> MVALSLKISIGNVVKTMQFEPSTMVYDACRIIRERIPEAPAGPPSDFGLFLSDDDPKKGIWLEAG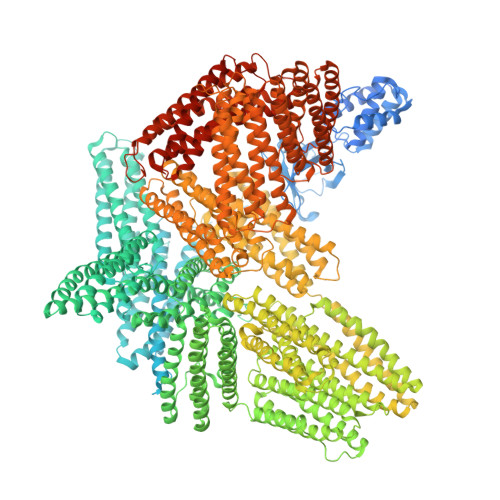KALDYYMLRNGDTMEYRKKQRPLKIRMLDGTVKTIMVDDSKTVTDMLMTICARIGITNHDEYSLVRELMEEKKEEITGTLRKDKTLLRDEKKMEKLKQKLHTDDELNWLDHGRTLREQGVEEHETLLLRRKFFYSDQNVDSRDPVQLNLLYVQARDDILNGSHPVSFDKACEFAGFQCQIQFGPHNEQKHKAGFLDLKDFLPKEYVKQKGERKIFQAHKNCGQMSEIEAKVRYVKLARSLKTYGVSFFLVKEKMKGKNKLVPRLLGITKECVMRVDEKTKEVIQEWNLTNIKRWAASPKSFTLDFGDYQDGYYSVQTTEGEQIAQLIAGYIDIILKKKKSKDHFGLEGDEESTMLEDSVSPKKSTVLQQQYNRVGKVEHGSVALPAIMRSGASGPENFQVGSMPPAQQQITSGQMHRGHMPPLTSAQQALTGTINSSMQAVQAAQATLDDFDTLPPLGQDAASKAWRKNKMDESKHEIHSQVDAITAGTASVVNLTAGDPAETDYTAVGCAVTTISSNLTEMSRGVKLLAALLEDEGGSGRPLLQAAKGLAGAVSELLRSAQPASAEPRQNLLQAAGNVGQASGELLQQIGESDTDPHFQDALMQLAKAVASAAAALVLKAKSVAQRTEDSGLQTQVIAAATQCALSTSQLVACTKVVAPTISSPVCQEQLVEAGRLVAKAVEGCVSASQAATEDGQLLRGVGAAATAVTQALNELLQHVKAHATGAGPAGRYDQATDTILTVTENIFSSMGDAGEMVRQARILAQATSDLVNAIKADAEGESDLENSRKLLSAAKILADATAKMVEAAKGAAAHPDSEEQQQRLREAAEGLRMATNAAAQNAIKKKLVQRLEHAAKQAAASATQTIAAAQHAASTPKASAGPQPLLVQSCKAVAEQIPLLVQGVRGSQAQPDSPSAQLALIAASQSFLQPGGKMVAAAKASVPTIQDQASAMQLSQCAKNLGTALAELRTAAQKAQEACGPLEMDSALSVVQNLEKDLQEVKAAARDGKLKPLPGETMEKCTQDLGNSTKAVSSAIAQLLGEVAQGNENYAGIAARDVAGGLRSLAQAARGVAALTSDPAVQAIVLDTASDVLDKASSLIEEAKKAAGHPGDPESQQRLAQVAKAVTQALNRCVSCLPGQRDVDNALRAVGDASKRLLSDSLPPSTGTFQEAQSRLNEAAAGLNQAATELVQASRGTPQDLARASGRFGQDFSTFLEAGVEMAGQAPSQEDRAQVVSNLKGISMSSSKLLLAAKALSTDPAAPNLKSQLAAAARAVTDSINQLITMCTQQAPGQKECDNALRELETVRELLENPVQPINDMSYFGCLDSVMENSKVLGEAMTGISQNAKNGNLPEFGDAISTASKALCGFTEAAAQAAYLVGVSDPNSQAGQQGLVEPTQFARANQAIQMACQSLGEPGCTQAQVLSAATIVAKHTSALCNSCRLASARTTNPTAKRQFVQSAKEVANSTANLVKTIKALDGAFTEENRAQCRAATAPLLEAVDNLSAFASNPEFSSIPAQISPEGRAAMEPIVISAKTMLESAGGLIQTARALAVNPRDPPSWSVLAGHSRTVSDSIKKLITSMRDKAPGQLECETAIAALNSCLRDLDQASLAAVSQQLAPREGISQEALHTQMLTAVQEISHLIEPLANAARAEASQLGHKVSQMAQYFEPLTLAAVGAASKTLSHPQQMALLDQTKTLAESALQLLYTAKEAGGNPKQAAHTQEALEEAVQMMTEAVEDLTTTLNEAASAAGVVGGMVDSITQAINQLDEGPMGEPEGSFVDYQTTMVRTAKAIAVTVQEMVTKSNTSPEELGPLANQLTSDYGRLASEAKPAAVAAENEEIGSHIKHRVQELGHGCAALVTKAGALQCSPSDAYTKKELIECARRVSEKVSHVLAALQAGNRGTQACITAASAVSGIIADLDTTIMFATAGTLNREGTETFADHREGILKTAKVLVEDTKVLVQNAAGSQEKLAQAAQSSVATITRLADVVKLGAASLGAEDPETQVVLINAVKDVAKALGDLISATKAAAGKVGDDPAVWQLKNSAKVMVTNVTSLLKTVKAVEDEATKGTRALEATTEHIRQELAVFCSPEPPAKTSTPEDFIRMTKGITMATAKAVAAGNSCRQEDVIATANLSRRAIADMLRACKEAAYHPEVAPDVRLRALHYGRECANGYLELLDHVLLTLQKPSPELKQQLTGHSKRVAGSVTELIQAAEAMKGTEWVDPEDPTVIAENELLGAAAAIEAAAKKLEQLKPRAKPKEADESLNFEEQILEAAKSIAAATSALVKAASAAQRELVAQGKVGAIPANALDDGQWSQGLISAARMVAAATNNLCEAANAAVQGHASQEKLISSAKQVAASTAQLLVACKVKADQDSEAMKRLQAAGNAVKRASDNLVKAAQKAAAFEEQENETVVVKEKMVGGIAQIIAAQEEMLRKERELEEARKKLAQIRQQQYKFLPSELRDEHLVVLFQ>ATQGVFTLPANTRFGVTAFANSSGTQTVNVLVNNETAATFSGQSTNNAVIGTQVLNSGSSGKVQVQVSVNGRPSDLVSAQVILTNELNFALVGSEDGTDNDYNDAVVVINWPLG[4x];>[2x]KYKKALKKLAKLL;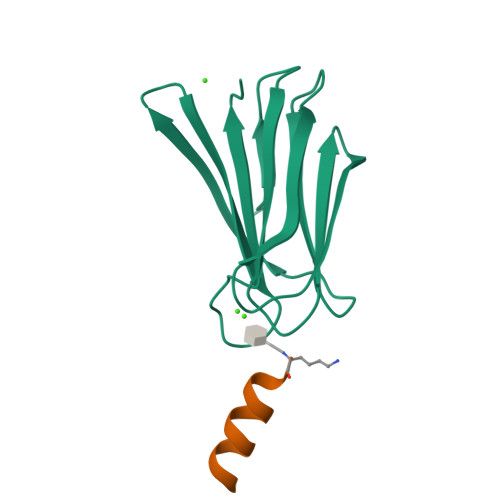>KYKKAL[2x]Bacteriophage Q protein has served as a paradigm for studying regulation of transcription elongation. Through its engagement with RNAP, Q renders RNAP resistant to terminators. The Q protein of bacteriophage 21 (21Q) was characterized as sharing a conserved mechanism of action with Q proteins from other lambdoid phages. To investigate how Q renders RNAP resistant to terminators, and to visualize sequence-specific interaction of Q with QBE, we determined a crystal structure of 21Q at 1.45 Å resolution and a single-particle cryo-electron microscopy (cryo-EM) structure of an intact 21Q-engaged arrested complex at 4.08 Å resolution.

The crystal structure of 21Q was determined at 1.45 Å resolution. The structure of 21Q contains six helices (H1-H6) and three long loops (L1-L3). A segment of L2 is disordered in the crystal structure, indicating the intrinsic flexibility of this region. Surprisingly, the structure of 21Q is reminiscent of the binary complex structure of σR4 bound to anti-σ RseA. Specifically, the folding of 21Q H3-H6 is similar to the folding of σR4, while 21Q H1 binds to 21Q H3-H6 in the same way as RseA binds to σR4. Because H3 and H4 of σR4 form a helix-turn-helix (HTH) motif and participate in the binding and recognition of the −35 element, the corresponding helices of 21Q (H5 and H6) probably participate in the binding and recognition of the QBE. Other than that, there is no structural similarity between 21Q and λQ, which is consistent with the observation that although both Q proteins act by a similar mechanism, there is no obvious homology to their protein sequences.

>MGIRELNLTKEQHEWLNGWLELWGAWVYSGRLEKRMSSVIAKFMESVEPGRVMTRPMCNDDDGMLISQVVDSVMYIDKKAFGILLSYYAHGSSKHAIASYYHRVARPRKMLCRGGGRIQKPSLATCRREVDEILNASLFMIYPVLDSAFKNRKRVEKIKHVA[2x]> SSYSGPIVVDPVTRIEGHLRIEVEVENGKVKNAYSSSTLFRGLEIILKGRDPRDAQHFTQRTCGVCTYTHALASTRCVDNAVGVHIPKNATYIRNLVLGAQYLHDHIVHFYHLHALDFVDVTAALKADPAKAAKVASSISPRKTTAADLKAVQDKLKTFVETGQLGPFTNAYFLGGHPAYYLDPETNLIATAHYLEALRLQVKAARAMAVFGAKNPHTQFTVVGGVTCYDALTPQRIAEFEALWKETKAFVDEVYIPDLLVVAAAYKDWTQYGGTDNFITFGEFPKDEYDLNSRFFKPGVVFKRDFKNIKPFDKMQIEEHVRHSWYEGAEARHPWKGQTQPKYTDLHGDDRYSWMKAPRYMGEPMETGPLAQVLIAYSQGHPKVKAVTDAVLAKLGVGPEALFSTLGRTAARGIETAVIAEYVGVMLQEYKDNIAKGDNVICAPWEMPKQAEGVGFVNAPRGGLSHWIRIEDGKIGNFQLVVPSTWTLGPRCDKNNV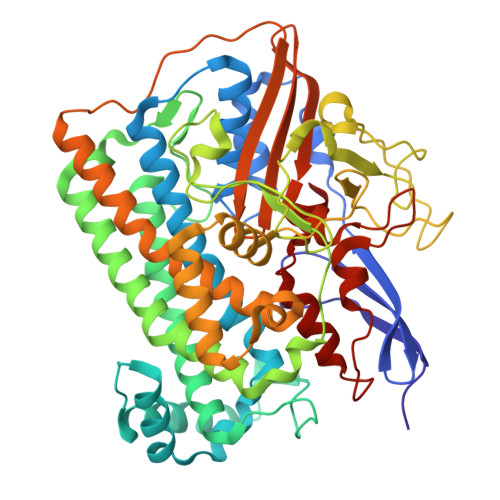SPVEASLIGTPVADAKRPVEILRTVHSFDPCIACGVH> MAKNRRDRNSWGGFSEKTYEWSSEEEEPVKKAGPVQVLIVKDDHSFELDETALNRILLSEAVRDKEVVAVSVAGAFRKGKSFLMDFMLRYMYNQESVDWVGDYNEPLTGFSWRGGSERETTGIQIWSEIFLINKPDGKKVAVLLMDTQGTFDSQSTLRDSATVFALSTMISSIQVYNLSQNVQEDDLQHLQLFTEYGRLAMEETFLKPFQSLIFLVRDWSFPYEFSYGADGGAKFLEKRLKVSGNQHEELQNVRKHIHSCFTNISCFLLPHPGLKVATNPNFDGKLKEIDDEFIKNLKILIPWLLSPESLDIKEINGNKITCRGLVEYFKAYIKIYQGEELPHPKSMLQATAEANNLAAVATAKDTYNKKME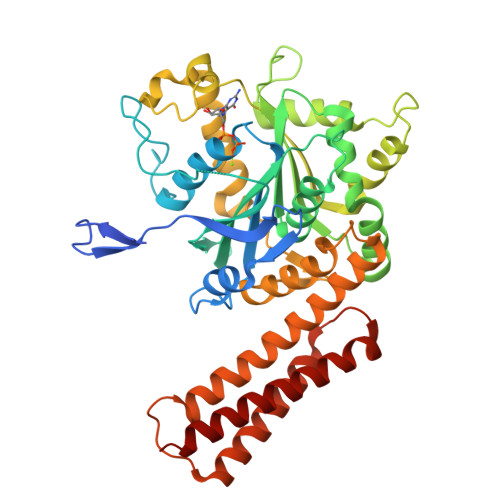EICGGDKPFLAPNDLQTKHLQLKEESVKLFRGVKKMGGEEFSRRYLQQLESEIDELYIQYIKHNDSK> AKLSCKICGYIYDEDE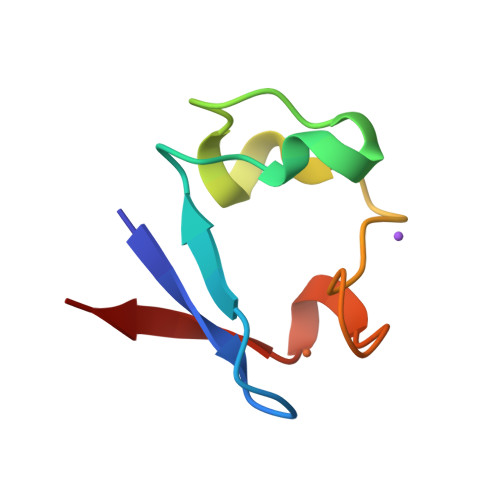GDPDNGISPGTKFEDLPDDWVCPLCGSPKSEFERIE>[2x]MAQAKHKQR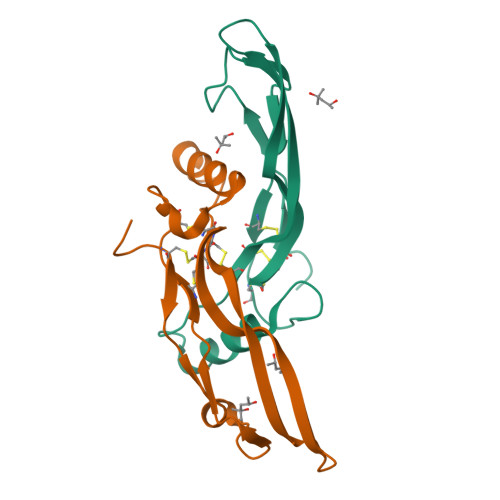KRLKACRKHELYVSFQDLGWQDWIIAPKGYAANYCDGECSFPLNAHMNATNHAIVQTLVHLMNPEYVPKPCCAPTKLNAISVLYFDDNSNVILKKYRNMVVRACGCH>[4x]MASMTGMPNYNIPFSPPDITEAEITEVVDTLRSGWITTGPKTKELERRLSLYTQTPKTVCLNSATAALELILRVLEVGPGDEVIVPAMTYTASCSVITHVGATPVMVDIQADTFEMDYDLLEQAITEKTKVIIPVELAGIVCDYDRLFQVVEKKRDFFTASSKWQKAFNRIVIVSDSAHALGSTYKGQPSGSIADFTSFSFHAVKNFTTAEGGSATWKANPVIDDEEMYKEFQILSLHGQTKDALAKMQLGSWEYDIVTPAYKCNMTDIMASLGLVQLDRYPSLLQRRKDIVDRYDSGFAGSRIHPLAHKTETVESSRHLYITRVEGASLEERNLIIQELAKAGIASNVHYKPLPLLTAYKNLGFDMTNYPKAYAFFENEITLPLHTKLSDEEVDYIIETFKTVSEKVLTLSKKKLAAALEHHHHHH

Spr1654 is involved in the early steps of TA precursor synthesis, where the first amino sugar UDP-AATGal is suggested to be synthesized by this aminotransferase, followed by several TA biosynthesis pathway steps. The three-dimensional structures revealed that Spr1654 has a fold characteristic of the type I aminotransferase family. Each Spr1654 subunit can be divided into an N-terminal arm (residues 1–14), a large PLP-binding domain comprising residues 15–276 and a smaller C-terminal domain comprising residues 277–404. Two dimers, composed of subunits AB and CD, are present in the asymmetric unit of all the obtained crystals of all forms of Spr1654, with a buried surface area of 2490 Å2 per monomer (15% of the total solvent accessible surface area).

The crystal structure of Spr1654 was determined in the apo-, PLP- and PMP-bound states at 1.9 Å, 2.2 Å and 2.4 Å resolutions, respectively. Consistent with the comparison between the apo- and ligand-bound forms of other SATs, nothing seems to happen with Spr1654 upon PLP/PMP dissociation. Indeed, the crystal structure of the apo-form of Spr1654 indicates that water molecules fill the cofactor-binding cavity, without any alteration of the conformation of any residue (data not shown). In all crystal structures, the electron density is well defined for residues Tyr4 to Thr404 within all the four subunits present in the asymmetric unit, except for a short helix comprising residues Ala238 to Leu244 that is missing due to flexibility in one subunit within each dimer (subunits B and D). This region of the protein could be part of the substrate-binding cleft, which explains its high mobility in the absence of substrate (see below).>[2x]GSPLLDDDDQVAFSFILDNIVTQKMMAVPDSWPFHHPVNKKFVPDYYKVIVNPMDLET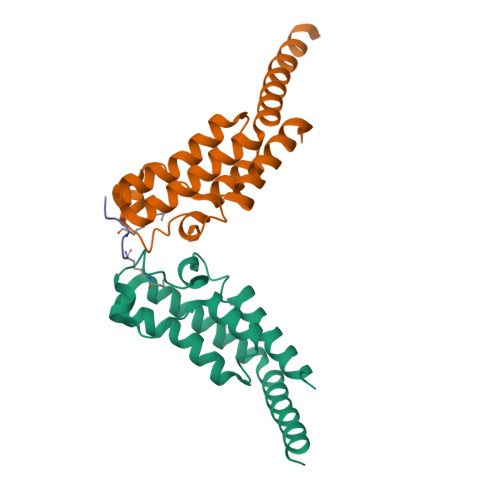IRKNISKHKYQSRESFLDDVNLILANSVKYNGPESQYTKTAQEIVNVCYQTLTEYDEHLTQLEKDICTAKEAALEEAELESLDPMT;> SGRGXGGXGLG> MGHHHHHHGDAALLLNVEGVKKTILHGGTGELPNFITGSRVIFHFRTMKCDEERTVIDDS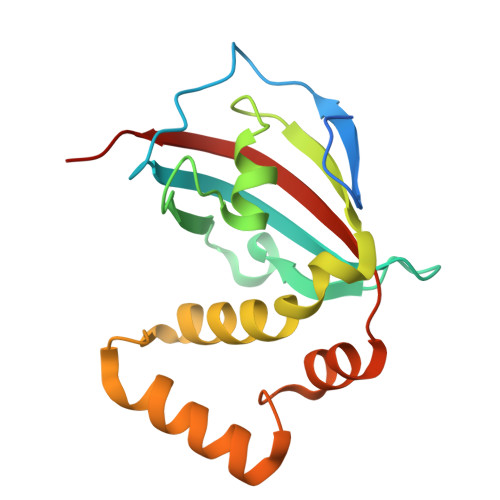RQVGQPMHIIIGNMFKLEVWEILLTSMRVHEVAEFWCDTIHTGVYPILSRSLRQMAQGKDPTEWHVHTCGLANMFAYHTLGYEDLDELQKEPQPLVFVIELLQVDAPSD Bunyamwera virus (BUNV) is the prototypic orthobunyavirus that serves as a tractable model for the Bunyavirales order. Each segment is encapsidated by multiple copies of the nucleocapsid protein (NP) to form a ribonucleoprotein (RNP), which associates with the virus-encoded RNA-dependent RNA polymerase (RdRp; L). RNPs serve as the active templates for all viral RNA synthesis activities and represent the form in which the RNA segments are packaged into virions. The BUNV NP comprises a globular core with N- and C-terminal lobes bisected by a positively charged RNA-binding groove, accommodating approximately 11 RNA bases.

Based on a cryo-EM average at 13 Å resolution and subsequent fitting of NP crystal structures by molecular dynamics, we were able to generate a pseudo-atomic model of the NP portion of the RNP. Given the absence of long, straight NP sections amenable to helical reconstruction, ~135,000 short NP sections were selected and processed using a single particle approach. Therefore, these numbers were applied for a final reconstruction with local searches, resulting in a 13 Å average that converged on a −105.26° twist and 18.25 Å rise. To preserve these aspects of the structure, we produced a model of what we termed ‘split’ NP that contained the core of a single NP monomer and the bound arms of its two neighbors. The NP structure was symmetrized, and molecular dynamics were applied to restrain the ‘split’ NP. This allowed freedom of movement of the linker region of each terminal arm, which had already been shown to be flexible while minimizing alterations to the globular core of the protein or the binding regions of the arms. A limitation of this approach was that it prevented us from modeling the viral RNA along the NP arms, and therefore, we did not include it in our model. Displaying the surface coulombic potential of the helical model confirms that the positively charged RNA-binding groove of each monomer is aligned in a way that maintains an RNA-binding channel along with the interior of the entire helical filament. Furthermore, these rungs were too far apart (approximately 18 Å) to permit intermolecular interactions of any kind between NP monomers along the longitudinal axis. Our model suggests that the helical arrangement of BUNV RNP is dictated by lateral NP-NP interactions and does not involve longitudinal NP-NP interactions, providing a molecular explanation of the RNP flexibility. However, by comparing these NP-NP contacts with those within the native helical NP, 7 novel residues were identified between laterally adjacent NP monomers with sidechains potentially involved in weak H-bond or salt bridge interactions within the RNP helix.

>[9x]MIELEFHDVAANTSSTFDPEVAYANFKRVHTTGLSYDHIRIFYIKGREIKTSLAKRSEWEVTLNLGGWKITVYNTNFPGNRNNPVPDDGLTLHRLSGFLARYLLEKMLKVSEPEKLIIKSKIINPLAEKNGITWNDGEEVYLSFFPGSEMFLGTFRFYPLAIGIYKVQRKEMEPKYLEKTMRQRYMGLEAATWTVSKLTEVQSALTVVSSLGWKKTNVSAAARDFLAKFGINM>[2x]MGEQVVKPTDERIIDPSTANTQLTGGVTYNTTSGGNKPLAGSPYGYETWIDTGGGVCSLTWYGADQGGGAAFKCTWTNPHDFLCRLGYFWNENKPYSHYENIYCGFNYTRSGRKTAGDYSYIGIYGWSRNPS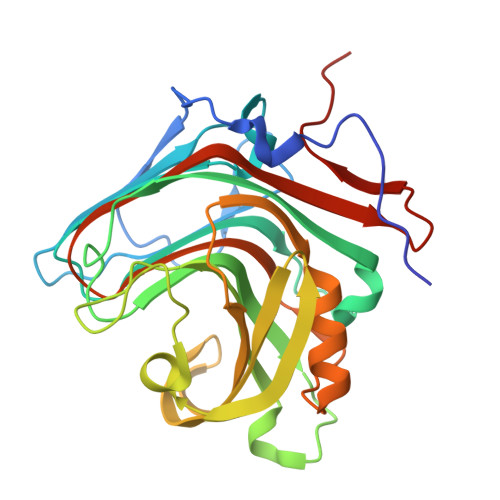ASNSNERLIEYYIVEDWFGNQWQADTSPMGINTTGGTVMGSFTVDGSSYQIIKNTRVNQPSIEGDKTFVQYFSIRQSPRKSGTISITEHFKKWEKLGMKLGDNMYECKFLIEAGAGEGFFDARLIQFYRADNEGNILQITPLEHHHHHH> EPFWADLQPRVAFVERGGSLWLNCSTNCPRPERGGLETSLRRNGTQRGLRWLARQLVDIREPETQPVCFFRCARRTLQARGLIRTFQRPDRVELMPLPPWQPVGENFTLSCRVPGAGPRASLTLTLLRGAQELIRRSFAGEPPRARGAVLTATVLARREDHGANFSCRAELDLRPHGLGLFENSSAPRELRTFSLSPDAPRLAAPRLLEVGSERPVSCTLDGLFPASEARVYLALGDQNLSPDVTLEGDAFVATATATASAEQEGARQLVCNVTLGGENRETRENVTIYSFPAPLLTLSEPSVSEGQMVTVTCAAGAQALVTLEGVPAAVPGQPAQLQLNATENDDRRSFFCD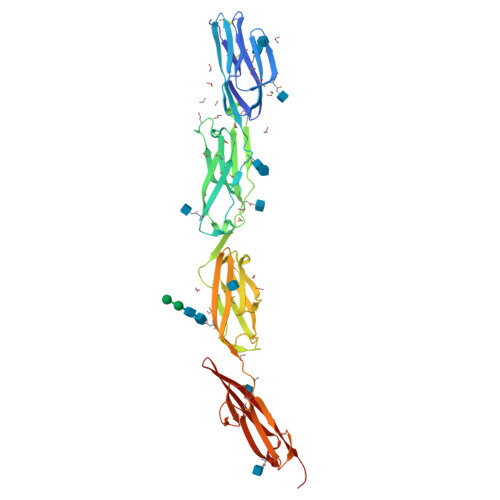ATLDVDGETLIKNRSAELRVLYAPR>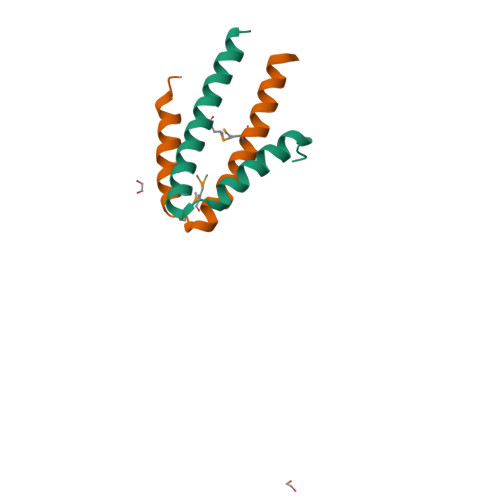MNQPIELSLEQQFSIRSFATQVQNMSHDQAKDFLVKLYEQMVVREATYQELLKHQWGLDSGSTPA[12x]>QKPGETKEVHPQLTTFRCTKRGGCKPATNFIVLDSLSHPIHRAEGLGPGGCGDWGNPPPKDVCPDVESCAKNCIMEGIPDYSQYGVTTNGTSLRLQHILPDGRVPSPRVYLLDKTKRRYEMLHLTGFEFTFDVDATKLPCGMNSALYLSEMHPTGAKSKYNPGGAYYGTGYCDAQCFVTPFINGLGNIEGKGSCCNSMDIWEANSRASHVAPHTCNKKGLYLCEGEECAFEGVCDKNGCGWNNYRVNVTDYYGRGEEFKVNTLKPFTVVTQFLANRRGKLEKIHRFYVQDGKVIESFYTNKEGVPYTNMIDDEFCEATGSRKYMELGATQGMGEALTRGMVLAMSIWWDQGGNMEWLDHGEAGPCA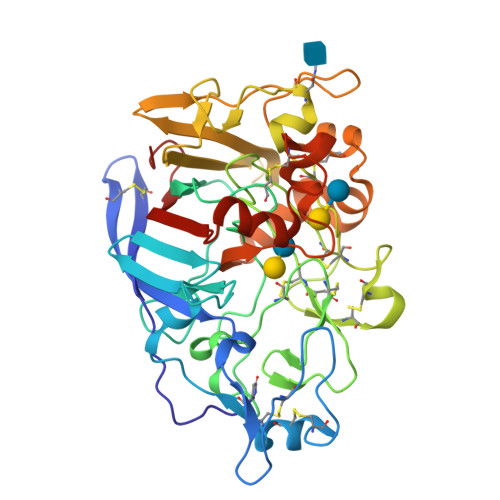KGEGAPSNIVQVEPFPEVTYTNLRWGEIGSTYQELQ[2x]>MSKRPNFLVIVADDLGFSDIGAFGGEIATPNLDALAIAGLRLTDFHTASAASPTRSMLLTGTDHHIAGLGTVAEALTPELEGKPGYEGHLNERVVALPELLREAGYQTLMAGKWHLGLKPEQTPHARGFERSFSLLPGAANHYGFEPPYDESTPRILKGTPALYVEDERYLDTLPEGFYSSDAFGDKLLQYLKERDQSRPFFAYLPFSAPHWPLQAPREIVEKYRGRYDAGPEALRQERLARLKELGLVEADVEAHPVLALTREWEALEDEERAKSARAMEVYAAMVERMDWNIGRVVDYLRRQG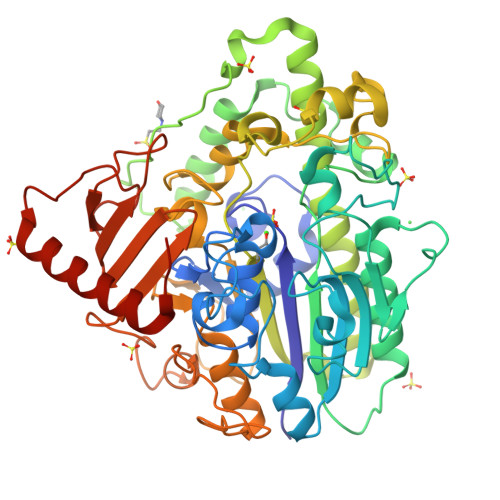ELDNTFVLFMSDNGAEGALLEAFPKFGPDLLDFLDRHYDNSLENIGSANSYVWYGPRWAQAATAPSRLYKAFTTQGGIRVPALVRYPRLSRQGAISHAFATVMDVTPTLLDLAGVRHPGKRWRGREIAEPRGRSWLGWLSGETEAAHDENTVTGWGLFGMRAIRQGDWKAVYLPAPVGPATWQLYDLARDPGEIHDLADSQPGKLAELIEHWKRYVSDTGVVEGASPFLVR[2x]>[2x]CCUCTGGTCTCC;>GG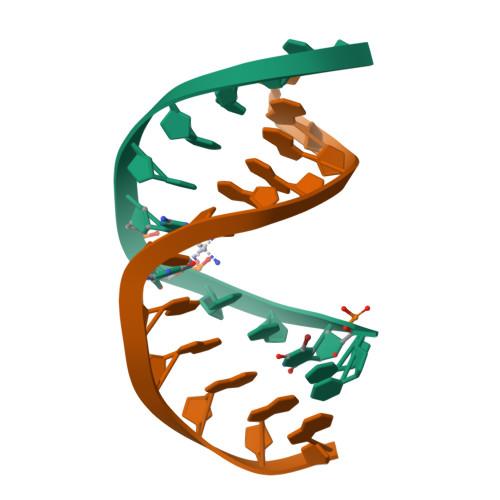AGACCAGAGG[2x]>SLANTYLLQDHNTLTPYTPFTTPLNGGLDVVRAAHLHPSYELVDWKRVGDTKLVALVRSALVRVKFQDTTSSDQSNTNQNALSFDTQESQKALNGSQSGSSDTSGSNSQDFASYVLIFKAAPRATWVFERKIKLALPYVKQESQGSGDQGSNGKGSLYKTLQDLLVEQPVTPYTPNAGLARVNGVAQDTVHFGSGQESSWNSQRSQKGLKNNPGPKAVTGFKLDKGRAYRKLNESWPVYEPLDSTKEGKGKDESSWKNSEKTTAENDAPLVGMVGSGAAGSASSLQGNGSNSSGLKSLLRSAPVSVPPSSTSNQTLSLSNPAPVGPQAVVSQPAGGATAAVSVNRTASDTATFSKYLNTAQALHQMGVIVPGLEKWGGNNGTGVVASRQDATSTNLPHAAGASQTGLGTGSPREPALTATSQRAVTVVAGPLRAGNSSETDALPNVITQLYHTSTAQLAYLNGQIVVMGSDRVPSLWYWVVGEDQESGKATWWAKTELNWGTDKQKQFVENQLGFKDDSNSDSKNSNLKAQGLTQPAYLIAGLDVVADHLVFAAFKAGAVGYDMTTDSSASTYNQALAWSTTAGLDSDGGYKALVENTAGLNGPINGLFTLLDTFAYVTPVSGMKGGSQNNEEVQTTYPVKSDQKATAKIASLINASPLNSYGDDGVTVFDALGLNFNFKLNEERLPSRTDQLLVYGIVNESELKSARENAQSTSDDNSNTKVKWTNTASHYLPVPYYYSANFPEAGNRRRAEQRNGVKISTLESQATDGFANSLLNFGTGLKAGVDPAPVARGHKPNYSAVLLVRGGVVRLNFNPDTDKLLDSTDKNSEPISFSYTPFGSAESAVDLTTLKDVTYIAESGLWFYTFDNGEKPTYDGKQQQVKNRKGYAVITVSRTGIEFNEDANTTTLSQAPAALAVQNGIASSQDDLTGILPLSDEFSAVITKDQTWTGKVDIYKNTNGLFEKDDQLSENVKRR[2x]

M. pneumoniae binds to host target cells by means of a polar structure known as the attachment organelle, and glides in the direction of this differentiated structure at a speed of ~1 µm/s. P1, together with the P40/P90 polypeptides, forms a transmembrane complex called the “Nap”. In the present work, we report the structures of M. pneumoniae proteins P1 and P40/P90 and of complexes of P40/P90 bound to sialylated oligosaccharides. The structural results reveal that P1 (1627 residues) and P40/P90 (1218 residues) present a similar overall organization and topology in the extracellular regions.

After numerous attempts, high-resolution diffracting crystals were grown from a construct, referred henceforth as P40/P90N, spanning residues Ser23-Val1003 that, by sequence alignment, corresponds to the N-terminal domain of the M. genitalium orthologous protein P110. The refined P40/P90N structure, at 2.65 Å resolution, has agreement R and Rfree factors of 21.4 and 23.4, respectively. The sequence of P40/P90N presents two long insertions with respect to P110 of more than 60 residues each (Gly297–Thr368 and Leu395–Thr462 that are referred as S1 and S2, respectively). Both insertions, completely disordered in the crystal structures determined, are found between β-propeller blades II and III. Besides insertions S1 and S2, the structure of P40/P90 presents only three short disordered loops (residues Ser118–Gly127, Ser168–Gly175, and Ala774–Arg777) and the N-terminal domain from P40/P90 can be seen as a well-defined globular structure with two long floppy pendants. The primary scission occurs between Arg445 and Ala446, located toward the C-end of insertion S2. Structural stability of the cleaved protein probably relies on the large interface between the P40 and P90 polypeptides, with 75 hydrogen bonds, 6 salt bridges, and a buried surface area of 10,480 Å2, which gives an estimated free energy of −55 kcal with an expected 100% probability of formation according to the Complexation Significance Score algorithm in PISA32. Regardless of the extend of proteolysis, all P40/P90N samples behave as a single and sharp peak by SEC–MALS indicating that cleavage takes place only when folding is completed and that a unique three-dimensional structure of P40/P90N is maintained.5-(1-benzyl-4-chloro-1H-imidazol-2-yl)-1,3-dimethylpyridin-2(1H)-one 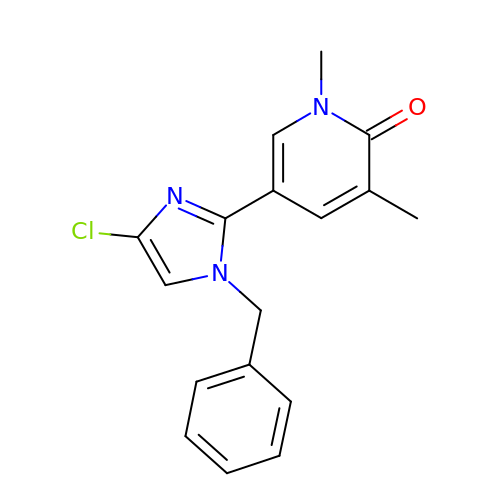| C17 H16 Cl N3 O | NCQBXRVQMFGJAV-UHFFFAOYSA-N Ca2+-ATPases transport calcium out of the cell or into internal stores and maintain a low concentration of free cytoplasmic calcium that can be four orders of magnitude below surroundings. Ca2+-ATPases encompass the P2A and P2B subtypes of the P-type family, consisting of typically ten membrane-spanning helical segments, M1-10, connected to three cytosolic domains: the nucleotide binding (N), the phosphorylation (P) with a catalytic aspartic acid residue conserved in all P-type ATPases, and the actuator (A) domain, which is involved in dephosphorylation and contains an essential TGES-motif containing loop. LMCA1 shares 34–39% sequence identity with mammalian SERCA (ATP2A genes), but it transports only a single calcium ion for each transport cycle, similar to the plasma membrane Ca2+-ATPase (PMCA, ATP2B genes) and the secretory pathway Ca2+-ATPase (SPCA, ATP2C genes) that share however a slightly lower sequence identity with LMCA1 (30-34%). P-type ATPases perform their active transport with energy from ATP hydrolysis via autoformation and breakdown of a phosphoenzyme and with structural transitions alternating between inward- and outward-oriented states.

We have determined a structure of the so far elusive calcium-occluded and ADP-insensitive [Ca]E2P intermediate for LMCA1 by cryo-EM using a G4 insertion mutant form, which is known to pause at this intermediate. To investigate G4-LMCA1 by cryo-EM, we incubated saposin-solubilized G4-LMCA1 with 1 mM Ca2+ and 1 mM ATP at room temperature for 2–10 min before plunge-freezing and cryo-EM imaging. We denote this state [Ca]E2P, as it displays features of both [Ca]E1P and E2P, with the TM domain adopting a calcium-bound conformation and the cytoplasmic domains assuming an E2P-like, ADP insensitive conformation. Further visual inspection reveals closed ion pathways, and density consistent with a single calcium ion bound and occluded at a binding site between M4 and M6, equivalent of SERCA site II. The calcium ion appears to coordinate two side chains in M6 (Asn716 and Asn720) and backbone carbonyl groups in M4 (Val287, Ala288, Ile290). However, the map for the [Ca]E2P form of G4-LMCA1 reveals no density for the Glu292 side chain oriented towards the calcium ion. The Glu292 residue of the calcium site appears flexible in the [Ca]E2P state (indicated by poor density and an orientation away from the Ca2+ site), and hence the calcium site has lower coordination by protein side chains, which may prime solvation of the Ca2+ ion and its release in the subsequent step. Phosphorylation of the catalytic aspartic acid residue in the P domain (Asp334 in LMCA1) is clearly visible (Fig. EV3), and the phosphorylation site is rotated away from the nucleotide-binding site of the N domain. Visual inspection of the cryo-EM density map indicates no density for bound nucleotide at the N domain despite a 1 mM background of ATP/ADP in the cryo-EM sample.

> MAEIYRKSAAETFTQLEATEKGLTTSEVTKRQEKYGFNELKNKKKGGGGDPLWKLFLETFKDPMVIVLVIAALVQLVLGEVVESLIIFLVLIVNSIISVVQTRKAESSLDALREMSAPVAKVIRDGSKQSIHARELVPGDVVILDAGDFVPADGRLFESGSLKIDEGMLTGESEAVEKYIDTIPDEVGLGDRVNMVFSGSLVVYGRGMFVVTGTASETEIGKIAGLLETAEAKQTPLQRKLESFSKKLGLGILALCVLIFAVEAGRVLLGDNSADMATAILNAFMFAVAVAVAAIPEALSSIVTIVLAVGTNKMAKQHAIIRKLPAVETLGSTSVICTDKTGTLTQNKMTVVDYYLPDGTKENFPESPENWSEGERRLIHIAVLCNDSNINSEGKELGDPTEVALIAFSNKNNQDYNEIREKFIREGEIPFDSDRKLMSTLHTFNENKAMLTKGGPDVMFARCSYVFLDGEEKPMTEEILAKLKETNEEFSNQALRVLAYGYKRMPADTTELKLEDEQDIVLVGLTAMIDPPREAVYASIEESKKAGIRTVMITGDHKTTAQAIGRDIGLMDADDIALTGQELDAMPEEELDKKLEHIAVYARVSPENKIRIVKAWQKKGKITAMTGDGVNDAPALKQADIGVAMGSGTDVAKDSAAMILTDDNFVSIVDAVGVGRTVFDNIKKSIAYLFAGNLGAIIAILFALVLDWINPFTALQLLFINLVNDSLPAIALGMEKAEPDVMKRKPRDINEGIFAGGTMRAVISRGVLIGIAVIISQYIGMQISPEMSVAMAFTTLILARTLQTFAARSNVQTAFGAGFFSNKYVIGAVLLCFVLYGITVLPGAREIFSIPASFGLHEWSIAAGLALAAVVMMEIIKVVQNKFFKDYDIPTTENLYFQGLEHHHHHHHHHH> MNIPQRQFSNEEVNRCYLRWQHLRNEHGMNAPSVPEFIYLTKVLQFAAKQRQELQMQRQQQGISGSQQNIVPNSSDQAELPNNASSHISASASPHLAPNMQLNGNETFSTSAHQSPIMQTQMPLNSNGGNNMLPQRQSSVGSLNATNFSPTPANNGENAAEKPDNSNHNNLNLNNSELQPQNRSLQEHNIQDSNVMPGSQINSPMPQQAQMQQAQFQAQQAQQAQQAQQAQQAQARLQQGRRLPMTMFTAEQSELLKAQITSLKCLVNRKPIPFEFQAVIQKSINHPPDFKRMLLSLSEFARRRQPTDQNNQSNLNGGNNTQQPGTNSHYNNTNTDNVSGLTRNAPLDSKDENFASVSPAGPSSVHNAKNGTLDKNSQTVSGTPITQTESKKEENETISNVAKTAPNSNKTHTEQNNPPKPQKPVPLNVLQDQYKEGIKVVDIDDPDMMVDSFTMPNISHSNIDYQTLLANSDHAKFTIEPGVLPVGIDTHTATDIYQTLIALNLDTTVNDCLDKLLNDECTESTRENALYDYYALQLLPLQKAVRGHVLQFEWHQNSLLTNTHPNFLSKIRNINVQDALLTNQLYKNHELLKLERKKTEAVARLKSMNKSAINQYNRRQDKKNKRLKFGHRLIATHTNLERDEQKRAEKKAKERLQALKANDEEAYIKLLDQTKDTRITHLLRQTNAFLDSLTRAVKDQQKYTKEMIDSHIKEASEEVDDLSMVPKMKDEEYDDDDDNSNVDYYNVAHRIKEDIKKQPSILVGGTLKDYQIKGLQWMVSLFNNHLNGILADEMGLGKTIQTISLLTYLYEMKNIRGPYLVIVPLSTLSNWSSEFAKWAPTLRTISFKGSPNERKAKQAKIRAGEFDVVLTTFEYIIKERALLSKVKWVHMIIDEGHRMKNAQSKLSLTLNTHYHADYRLILTGTPLQNNLPELWALLNFVLPKIFNSVKSFDEWFNTPFANTGGQDKIELSEEETLLVIRRLHKVLRPFLLRRLKKDVEKELPDKVEKVVKCKMSALQQIMYQQMLKYRRLFIGDQNNKKMVGLRGFNNQIMQLKKICNHPFVFEEVEDQINPTRETNDDIWRVAGKFELLDRILPKLKATGHRVLIFFQMTQIMDIMEDFLRYINIKYLRLDGHTKSDERSELLRLFNAPDSEYLCFILSTRAGGLGLNLQTADTVIIFDTDWNPHQDLQAQDRAHRIGQK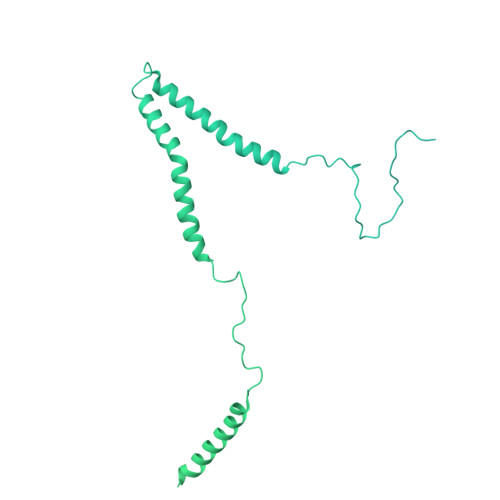NEVRILRLITTNSVEEVILERAYKKLDIDGKVIQAGKFDNKSTSEEQEALLRSLLDAEEERRKKRESGVEEEEELKDSEINEILARNDEEMAVLTRMDEDRSKKEEELGVKSRLLEKSELPDIYSRDIGAELKREESESAAVYNGRGARERKTATYNDNMSEEQWLRQFEVSDDEKNDKQARKQRTKKEDKSEAIDGNGEIKGENIDADNDGPRINNISAEDRADTDLAMNDDDFLSKKRKAGRPRGRPKKVKLEGSENSEPPALESSPVTGDNSPSEDFMDIPKPRTAGKTSVKSARTSTRGRGRGRGRGRGRGRGRGRPPKARNGLDYVRTPAAATSPIDIREKVAKQALDLYHFALNYENEAGRKLSDIFLSKPSKALYPDYYMIIKYPVAFDNINTHIETLAYNSLKETLQDFHLIFSNARIYNTEGSVVYEDSLELEKVVTKKYCEIMGDNSQLDFTEFDEQYGTRPLVLPPVVTSSVAESFTDEADSSMTEASV> MTMSVADAHALIKTIPDFPTKGIAFKDLSDILSTPAALDAVRKEVTAHYKDVPITKVVGIESRGFILGGIVANSLGVGFVALRKAG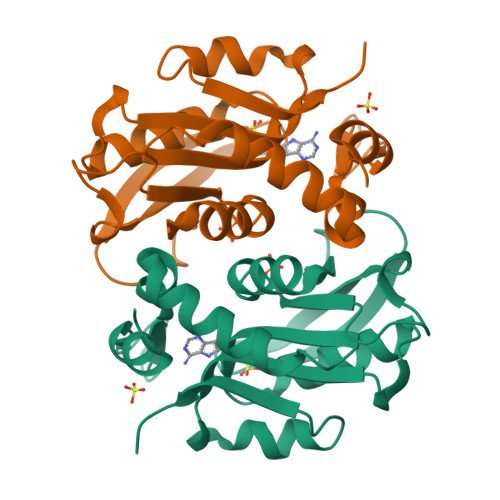KLPGDVCKCTFDMEYQKGVTIEVQKRQLGPHDVVLLHDDVLATGGTLLAAIELCETAGVKPENIYINVLYEIEALKGREKVGQKCTRLFSVIREHHHHHH> GPLGSNNMIGEIENRSTFL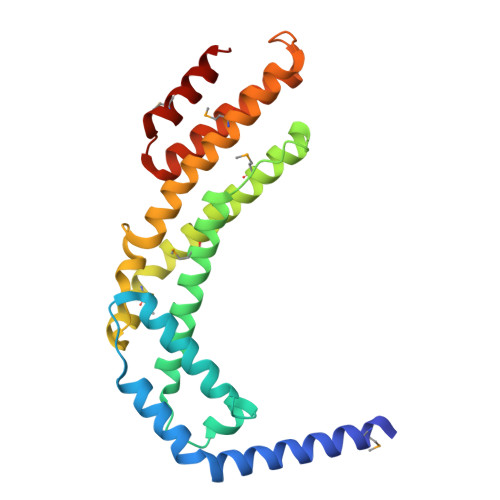LAVKADVETQGDFVQSLATEVRASSFTDIEDLLAFVSWLDEELSFLVDERAVLKHFDWPEGKADALREAAFEYQDLMKLEKQVTSFVDDPNLSSEPALKKMYKLLEKVEQSVYALLRTRDMAISRYKEFGIPVDWLSDTGVVGKIKLSSVQLAKKYMKRVAYELDSVSGSDKDPNREFLLLQGVRFAFRVHQFAGGFDAESMKAFEELRSRA>[2x]VVGGEDAKPGQFPWQVVLNGKVDAFCGGSIVNEKWIVTAAH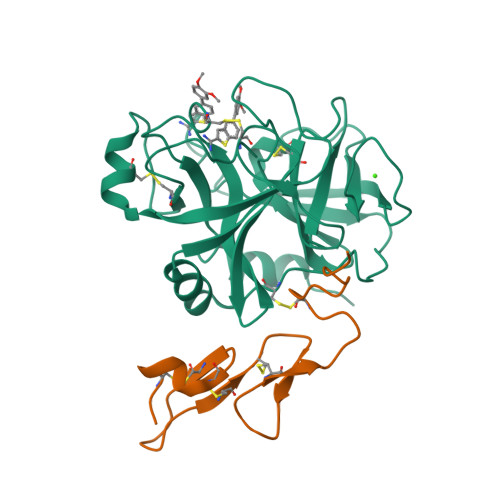CVETGVKITVVAGEHNIEETEHTEQKRNVIRIIPHHNYNAAINKYNHDIALLELDEPLVLNSYVTPICIADKEYTNIFLKFGSGYVSGWGRVFHKGRSALVLQYLRVPLVDRATCLRSTKFTIYNNMFCAGFHEGGRDSCQGDSGGPHVTEVEGTSFLTGIISWGEECAMKGKYGIYTKVSRYVNWIKEKTKLT;>[2x]MTCNIKNGRCEQFCKNSADNKVVCSCTEGYRLAENQKSCEPAVPFPCGRVSVSQTSK> IVGGTNSSWGEWPWQVSLQVKLTAQRHLCGGSLIGHQWVLTAAHCFDGLPLQDVWRIYSGILNLSDITKDTPFSQIKEIIIHQNYK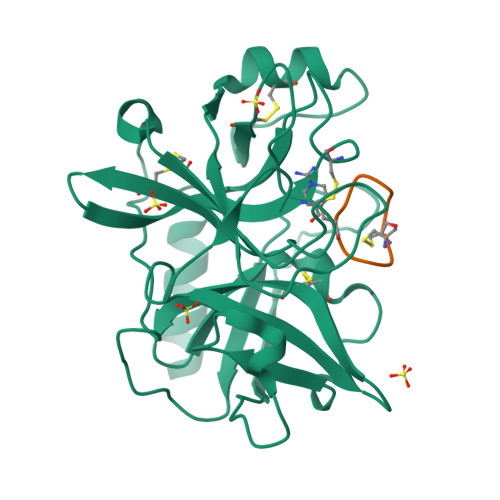VSEGNHDIALIKLQAPLNYTEFQKPISLPSKGDTSTIYTNCWVTGWGFSKEKGEIQNILQKVNIPLVTNEECQKRYQDYKITQRMVCAGYKEGGKDACKGDSGGPLVCKHNGMWRLVGITSWGEGCARREQPGVYTKVAEYMDWILEKTQSSD;> CPKRFAALFC>[4x]MNRSALDFRHFVDHLRRQGDLVDVHTEVDANLEIGAITRRVYERR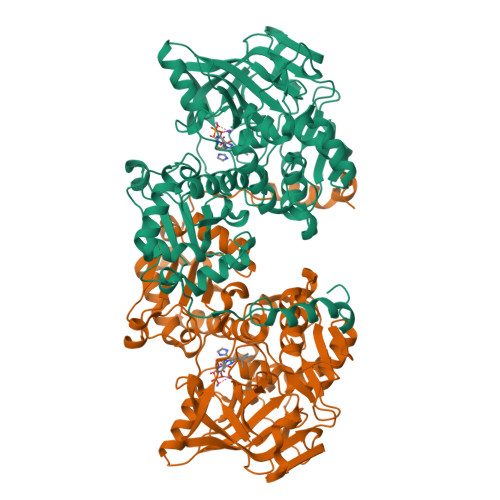APAPLFHNIRDSLPGARVLGAPAGLRADRARAHSRLALHFGLPEHSGPRDIVAMLRAAMRAEPIAPRRLERGPVQENVWLGEQVDLTRFPVPLLHEQDGGRYFGTYGFHVVQTPDGSWDSWSVGRLMLVDRNTLAGPTIPTQHIGIIREQWRRLGKPTPWAMALGAPPAALAAAGMPLPEGVSEAGYVGALVGEPVEVVRTQTNGLWVPANTEIVLEGEISLDETALEGPMGEYHGYSFPIGKPQPLFHVHALSFRDQPILPICVAGTPPEENHTIWGTMISAQLLDVAQNAGLPVDMVWCSYEAATCWAVLSIDVQRLAALGTDAAAFAARVAETVFGSHAGHLVPKLILVGNDIDVTEIDQVVWALATRAHPLHDHFAFPQIRDFPMVPYLDAEDKARGSGGRLVINCLYPEQFAGQMRAATASFRHAYPTALRRRVEERWSDYGFGDA>GSHMIWEQHTVTLHRAPGFGFGIAISGGRDNPHFQSGETSIVISDVLKGGPAEGQLQENDRVA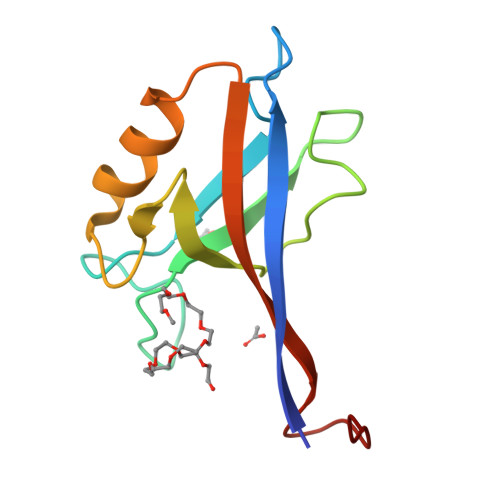MVNGVSMDNVEHAFAVQQLRKSGKNAKITIRRKKGGGSSGKDYV[2x]>LEVGRNSPYDYRIKSVVYNPVNVVKIDAVAGVATHIVVAPDETYITHAFGDSESRTFAHKMNHFFVKPKQAMSDTNLVIVTDKRTYNIVLHFIGEETKKNADGTVS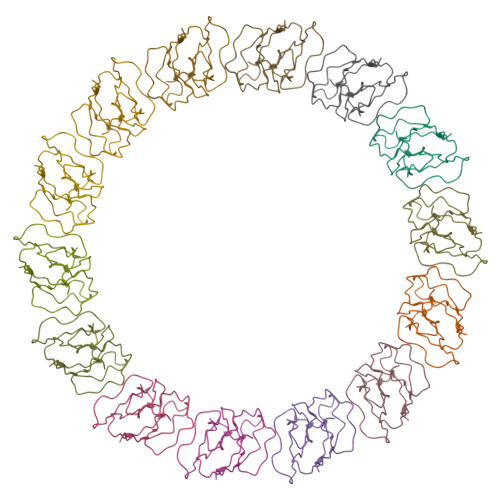KSFIET[14x]> AQYEDGKQYTTLEKPVAGAPQVLEFFSFFCPHAYQFEEVLHISDNVKKKLPEGVKMTKYHVNFMGGDLGKDLTQAWAVAMALGVEDKVTVPLFEGVQKTQTIRSASDIRDVF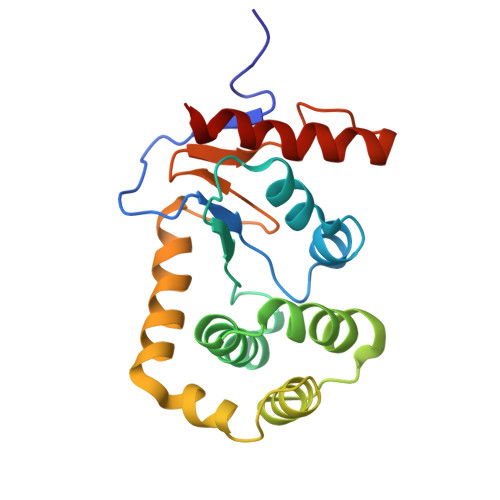INAGIKGEEYDAAWNSFVVKSLVAQQEKAAADVQLRGVPAMFVNGKYQLNPQGMDTSNMDVFVQQYADTVKYLSEKK> VRLPGLAAMRQGTRLFTPEQGEDLREALRRRRGSFQTTCEVTSETTFAAARRLREKASALAALNFASAKNPGGGFLGGAQAQEEDLCRGSGLYFSLTSPQAEPYYAVNRQSHSALYTDHLIYSPQVPIFRDDAGQLLPAPVPVNIITAPAPNAGAVAQSRPEQLPQVLPTLRERARRVLGVAAW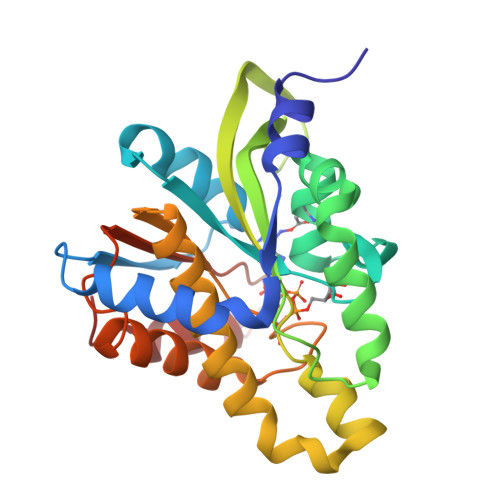MEQTHLVLGAWGCGVFRNDPAGVARTFRELLEGEAQGAFEHVTFAVLDNHPQHPTLGAFRRELESLC> GSGEADMDFLRNLFSQTLSLGSQKERLLDELTLEGVARYMQSERCRRVICLVGAGISTSAGIPDFRSPSTGLYDNLEKYHLPYPEAIFEISYFKKHPEPFFALAKELYPGQFKPTICHYFMRLLKDKGLLLRCYTQNIDTLERIAGLEQEDLVEAHGTFYTSHCVSASCRHEYPLSWMKEKIFSEVTPKCEDCQSLVKPDIVFFGESLPARFFSCMQSDFLKVDLLLVMGTSLQVQPFASLISKAPLSTPRLLINKEKAGQSDPFLGMIMGLGGGMDLGETPFDDIATFDSKKAYRDVAWLGECDQGCLALAELLGWKKELEDLVRREHASIDAQS

Sirtuin 2 (SIRT2), a member of the NAD+-dependent histone deacetylase family, has recently received increasing attention due to its potential involvement in neurodegenerative diseases and the progression of cancer. Human sirtuins (SIRT1–7) are currently the only known class of histone deacetylases that require NAD+ to catalyze the selective deacetylation of lysine in histone and non-histone proteins. The catalytic region of sirtuins consists of a Rossmann-fold domain, a zinc-binding domain and the loops connecting them. The interface between the loops and the two domains form both NAD+ (subdivided by the pockets A–C) and Ac-Lys substrate-binding sites.

Herein, with the aim to elucidate the binding mode of this prototype and to further improve the inhibitory activity, we initially solved the single-crystal X-ray diffraction structure of SIRT2 in complex with 3′-phenethyloxy-2-anilinobenzamide, which revealed that 6 is located in the selectivity pocket. The inhibitor binds to a highly lipophilic pocket localized at the interface between the Rossmann-fold domain and a small domain adjacent to the C-pocket of the NAD+-binding site. The binding mode analysis of 6 revealed that its phenoxyethylphenyl moiety is surrounded by Phe131, Leu134, Leu138, Tyr139, Pro140, Phe143 and Ile169, which leads to the establishment of π–π and H–π interactions. The 2-aminobenzamide moiety oriented towards the acetyl–lysine tunnel exhibits hydrogen bonds with water molecules HOH3, HOH4 and HOH11. Of these three water molecules, HOH3 and HOH4 are stabilized by a hydrogen bond network with the side chain of the catalytically active His187 and the main chain of Val233, i.e., the key amino acid residues that stabilize the binding of the acetyl–lysine substrate during the deacetylation reaction. Closer evaluation of the superimposed SIRT2 structures revealed that the amide group of 6 might occupy the same space as the methyl group of the N ε-acetyl–lysine substrate. This result prompted us to take a new perspective toward targeting the substrate-binding site through the functionalization of the benzamide moiety in 6 to mimic the acetyl–lysine interactions, which afforded compounds 17–19, 26–28, 36, 41 and 42. In the field of SIRT2 inhibitor design, a milestone on the elucidation of the mechanism behind the isotype selectivity of SIRT2 inhibitors has recently been reported by Rumpf et al., who discovered that the novel drug-like small molecule SirReal2 (5)32,33 is able to induce a rearrangement of the SIRT2 active site by creating a binding pocket, called the “selectivity pocket”, which is responsible for isoform specificity, suggesting a potential common mode of action for selective SIRT2 inhibitors. In fact, the “selectivity pocket” is the pocket that accommodates the long chain fatty acyl groups. In this study, the binding mode of 6 on SIRT2 was elucidated using X-ray crystallography.>SNESVDYRATFPE[2x];>GSLIGLMKDAFQPHHHHHHHLSPHPPGTVDKKMVEKCWKLMDKVVRLCQNPKLALKNSPPYILDLLPDTYQHLRTILSRYEGKMETLGENEYFRVFMENLMKKTKQTISLFKEGKERMYEENSQPRRNLTKLSLIFSHMLAELKGIFPSGLFQGDTFRITKADAAEFWRKAFGEKTIVPWKSFRQALHEVHPISSGLEAMALKSTIDLTCNDYISVFEFDIFTRLFQPWSSLLRNWNSLAVTHPGYMAFLTYDEVKARLQ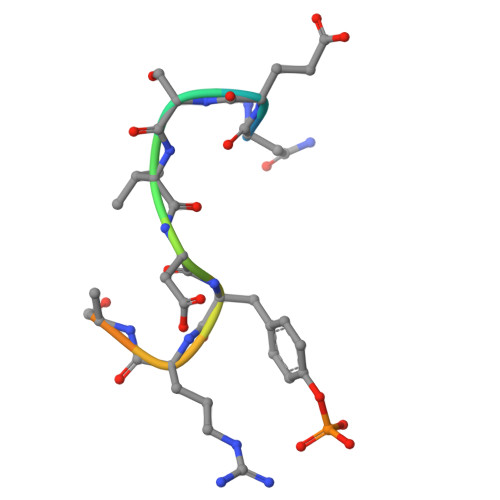KFIHKPGSYIFRLSCTRLGQWAIGYVTADGNILQTIPHNKPLFQALIDGFREGFYLFPDGRNQNPDLTG[2x]>AVNQSSSVEVSSESYETIFSQRIIRDLQKELVVGALFEELPMSSKILTMLVEPDAGKATWVAASTYGTDTTTGEEVKGALKEIHFSTYKLAAKSFITDETEEDAIFSLLPLLRKRLIEAHAVSIEEAFMTGDGSGKPKGLLTLASEDSAKVVTEAKADGSVLVTAKTISKLRRKLGR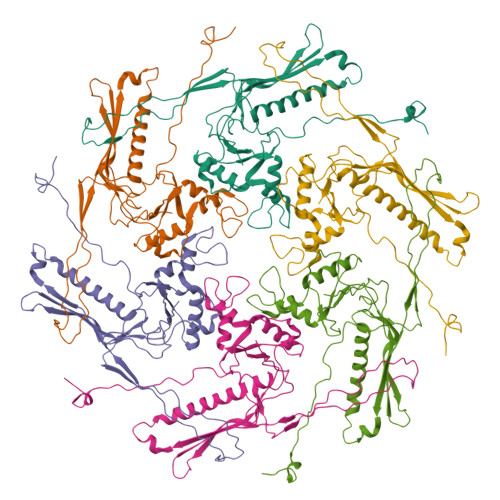HGLKLSKLVLIVSMDAYYDLLEDEEWQDVAQVGNDSVKLQGQVGRIYGLPVVVSEYFPAKANSAEFAVIVYKDNFVMPRQRAVTVERERQAGKQRDAYYVTQRVNLQRYFANGVVSGTYAAS[6x]> MASSKAKLEEIPITVDFSGGLEMLFDNQRRHSISLPAKDTEGKPVTIAFLIDYISKKLMK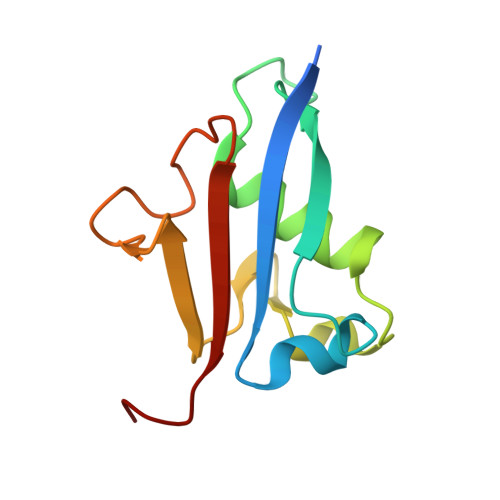DPRTDLFVLDNHIRPGILVLINDADWELEGEEAYEIQPNDNILFVSTLHGG> MAFEALTGINGDLITRSWSASKQAYLTERYHKEEAGAVVIFAFQPSFSEKDFFDPDNKSSFGEIKLNRVQFPCMRKIGKGDVATVNEAFLKNLEAIIDPRTSFQASVEMAVRSRKQIVFTGHSSGGATAILATVWYLEKYFIRNPNVYLEPRCVTFGAPLVGDSIFSHALGREKWSRFFVNFVSRFDIVPRIMLARKASVEETLPHVLAQLDP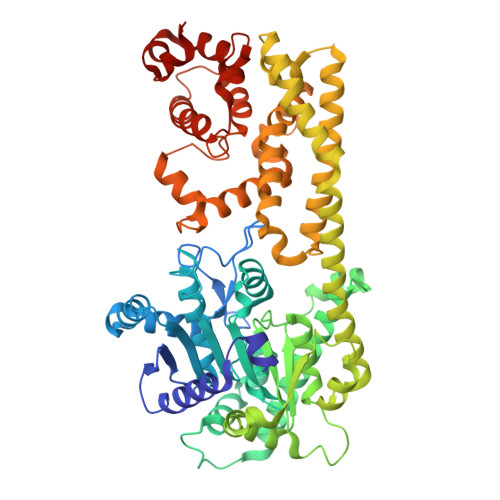RKSSVQESEQRITEFYTRVMRDTSTVANQAVCELTGSAEAFLETLSSFLELSPYRPAGTFVFSTEKRLVAVNNSDAILQMLFYTSQASDEQEWSLIPFRSIRDHHSYEELVQSMGKKLFNHLDGENSIESTLNDLGVSTRGRQYVQAALEEEKKRVENQKKIIQVIEQERFLKKLAWIEDEYKPKCQAHKNGYYDSFKVSNEENDFKANVKRAELAGVFDEVLGLMKKCQLPDEFEGDIDWIKLATRYRRLVEPLDIANYHRHLKNEDTGPYMKRGRPTRYIYAQRGYEHYILKPNGMIAEDVFWNKVNGLNLGLQLEEIQETLKNSGSECGSCFWAEVEELKGKPYEEVEVRVKTLEGMLGEWITDGEVDDKEIFLEGSTFRKWWITLPKNHKSHSPLRDYMMDEITDT> ENLLLRYL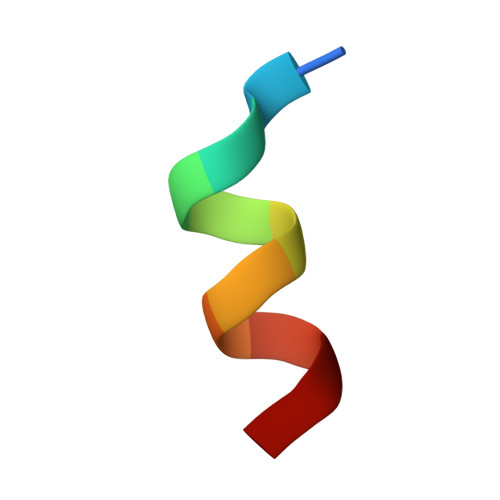LDK>SMSNRLIFDADWLVPEQVQVAGQAIQYYAARNIQYVQHPVAAIQVLNVFVPAAYLHGSSVNGYQRATAPILMPNTVGGYLPGPADDPQRVTWPTNAGTIQQALKRGYVVVAAGIRGRTTVDKSGQRVGQAPAFIVDMKAAIRYVKYNQGRLPGDANRIITNGTAAGGATSALAGASGNSAYFEPALTALGAAPATDDIFAVSAYCPIHNLEHADMAYEWQFNGINDWHRYQPVAGTTKNGRPKFEPVSGQLTVEEQALSLALKAQFSTYLNQLKLTASDGTHLTLNEAGMGSFRDVVRQLLISSAQTAFDQGTDIHKYAGFVVTGNQVTDLDLSAYLKSLTRMKA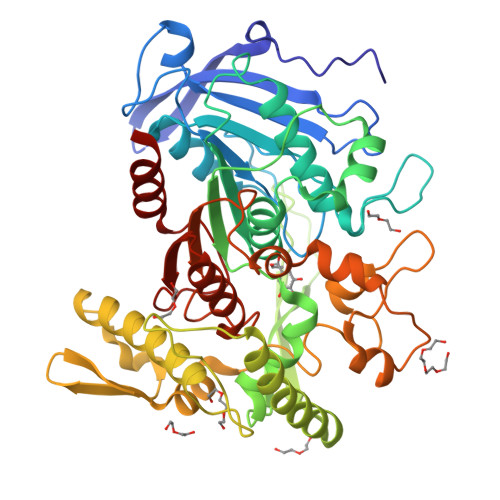VPAFDQLDLTSPENNLFGDATAKAKHFTALAQTRSTVTAQLADAELIQAINPLSYLTTTSSQVAKHWRIRHGAADRDTSFAIPIILAIMLENHGYGIDFALPWDIPHSGDYDLGDLFSWIDGLCQ[2x]>MFERIDYYAGDPILGLVEKFAADNNPDKVNLGIGIYYDESGVMPVLDCVKIAEQRIADPISPRPYLPMAGLPGHRKGCQELLFGKDAPVLKDGLVATIATIGGSGALKVGAEFIHEWFPQSKCYVSDPTWGNHIAIFEGCDIEVGKYPYYDTATGGIKFDEMIAFFETLNKDDVLLLHPCCHNPTGVDLTREQWDTVLNVIQERELIPFMDIAYQGFGEDMDSDAYAIRKAVDMGLPLFVSNSFSKNLSLYGERVGGLSVVCPTVDETERVFGQLNSTVRRIYSSPPSHGGRVVDIVMNDAALHEQWVGEVYAMRDRIKSMRTKLKSVLEAKISGRNFDYLTAQNGMFSFTGLTPEQVERLQSEFGIYMISNSRMCVAGLNSSNIDYVANAMVDVLKD[4x]

The psychrophilic aromatic aminotransferase from Psychrobacter sp. B6 is a representative of pyridoxal phosphate (PLP)-dependent enzymes. PsyArAT exhibits an activity typical for ArAT: transamination, which is a transfer of an amine group between aromatic α-amino acids and α-ketoacids. The mechanism of active site adjustment toward substrates of psychrophilic aromatic amino acid aminotransferase (PsyArAT) from Psychrobacter sp. B6 is discussed based on crystal structures of complexes with four hydroxy-analogs of substrates: phenylalanine, tyrosine, tryptophan and aspartic acid. These competitive inhibitors are bound in the active center of PsyArAT but do not undergo transamination reaction, which makes them an outstanding tool for examination of the enzyme catalytic center.

PsyArAT/WOH was another complex with different crystallographic properties, as it crystallized in a C2 group as a double dimer with noncrystallographical symmetry. In PsyArAT/WOH, PLP was added to the crystallization solution, which helped to obtain very good electron density maps for the cofactor. Tryptophan hydroxy-analog (WOH) created a network of contacts, enabling the involvement of both termini and a large domain, which resulted in closure conformation. High similarity of interactions with an inhibitor in catalytic centers of monomers A and C allowed for the description of only one of them, and we arbitrary choose monomer A. The carboxylic group of the WOH is planar to the Arg374 guanidine group, and two hydrogen bonds of 3.2 Å and 2.9 Å are made between them. The another contact in the length of 2.4 Å, of the mentioned carboxyl group, was made with the peptide bond hydrogen of Gly34, being part of the motile, long entrance loop. Additionally, side chain nitrogen atoms of Trp130 and Asn183, from the large domain, make hydrogen bonds (3.4 Å and 3.2 Å) with the carboxyl group of the ligand. Internal aldimine present in the catalytic center interacts with the carboxyl group of the WOH; the bond between the Schiff base nitrogen and oxygen atom is 3.2 Å long. Like in the case of the remaining complexes with aromatic ligands, FOH and YOH, Arg280*, from the second monomer, is in the “down” position, and one of its terminal nitrogen atoms creates two hydrogen bonds with side chains of Tyr8 and Asp11 (3.2 Å and 2.6 Å). Interestingly, in the active site of monomer A and C in the PsyArAT/WOH complex, the presence of a big, hydrophobic indole group of the WOH molecule, just near the Arg280* residue, prevented its contact with the Asn132 side chain (which was pushed away from the active pocket). Baffling was a lack of WOH in one monomer of each dimer in PsyArAT/WOH, which resulted in a huge difference in the volume of the active pocket, with the tryptophan hydroxy-analog present or absent in the active center.> PVSVPYSSAQ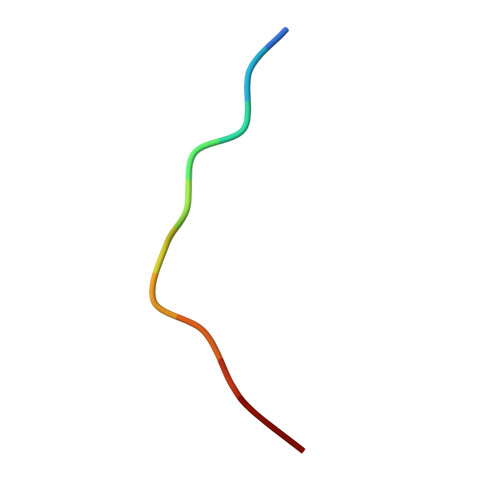S>MNREEMTLLGFEIVAYAGDARSKLLEALKA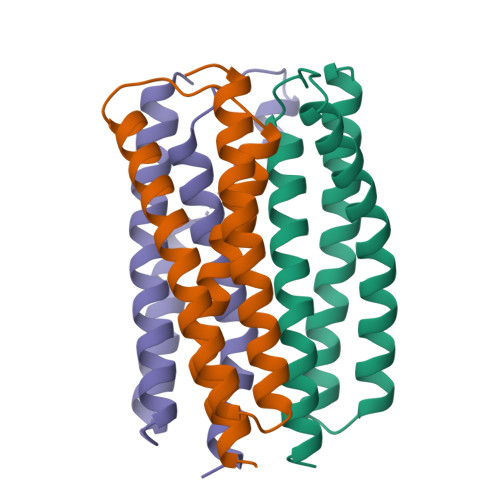AENGDFAKADSLVVEAGSCIAEAHSSQTGMLAREASGEELPYSVTMMHGQLHLMTTILLKDVIHHLIELYKRGAK[3x]>MSLNRHFTVSVFIVCKDKVLLHLHKKAK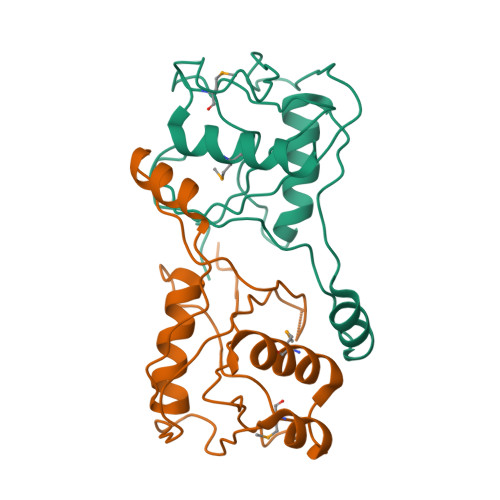KMLPLGGHIEVNELPEEACIREAKEEAGLNVTLYNPIDINLKKSCDLSGEKLLINPIHTILGDVSPNHSHIDFVYYATTTSFETSPEIGESKILKWYSKEDLKNAHNIQENILVMATEALDLLEGHHHHHH[2x]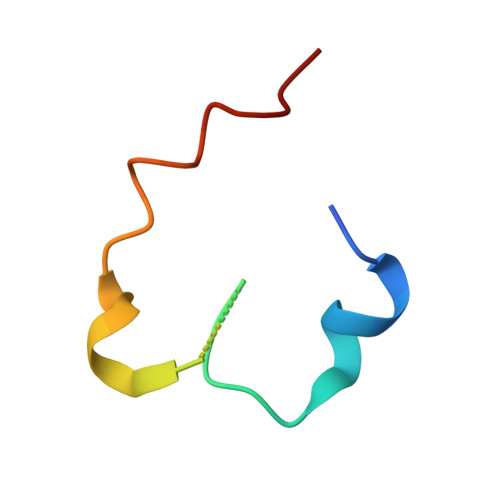> MFDTNATRLPIWGIGCNPWTAEHVDQTLASGNDIC>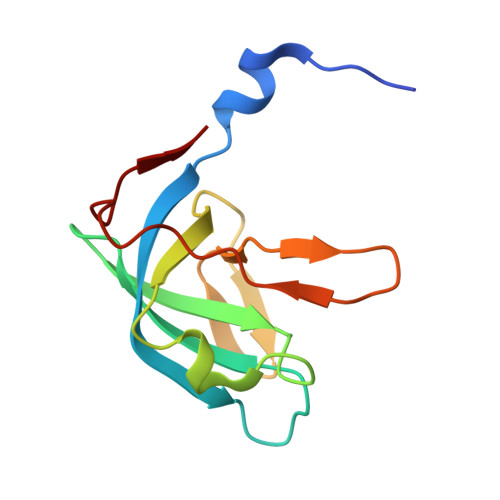 MNYMELYDVDEFWKFQMKVGLVKKAEKIKRTKKLIKLIVDFGNEERTIVTGIADQIPPEELEGKKFIFVVNLKPKKFSGVESQGMLILAETEDGKVYLIPVPEEVPVGARVW>[2x]MNVDILKQRAKAFDYVFDAIVVTDLQGFIIDWNKGSETLY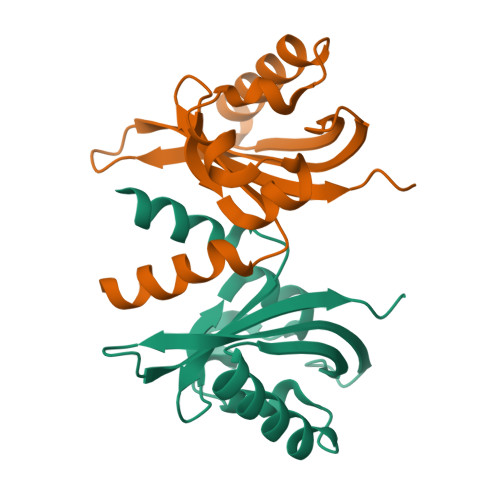GYSKEQAIGQPVNMLHVPGDTEHITSEVISAVENQGKWTGEIRMLHKDGHIGWIESMCVPIYGENYQMVGALGINRDITKRKKE> GSHTAEEDMEDDTSWRSEATFQFTVERFSRLSESVLSPPCFVRNLPWKIMVMP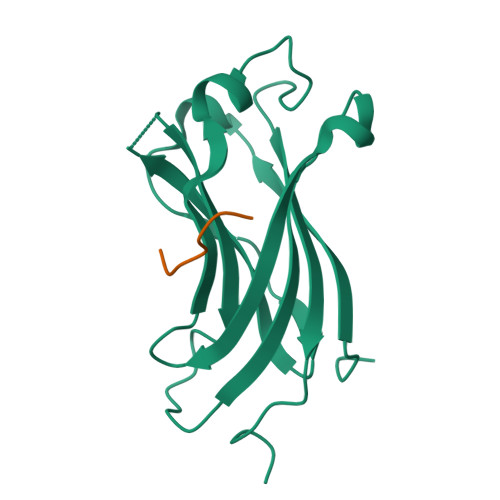RFYPDRPHQKSVGFFLQCNAESDSTSWSCHAQAVLKIINYRDDEKSFSRRISHLFFHKENDWGFSNFMAWSEVTDPEKGFIDDDKVTFEVFVQADAPHGVAW;> GARAHSS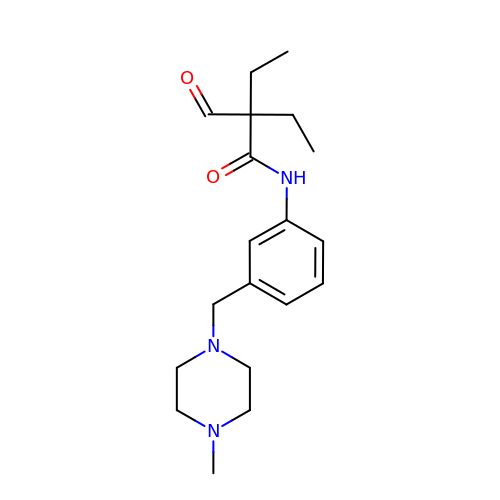2-ethyl-2-methanoyl-~{N}-[3-[(4-methylpiperazin-1-yl)methyl]phenyl]butanamide | C19 H29 N3 O2 | PBQJLTCTNSPMSB-UHFFFAOYSA-N> EGLEQLEAQTNFTKRELQVLYRGFKNECPSGVVNEDTFKQIYAQFFPHGDASTYAHYLFNAFDTTQTGSVKFEDFVTALSILLRGTVHEKLRWTFNLYDINKDGYINKEEMMDIVKAIYDMMGAYTYPVLAEDTPRQHVDVFFQKMDKNKDGIVTLDE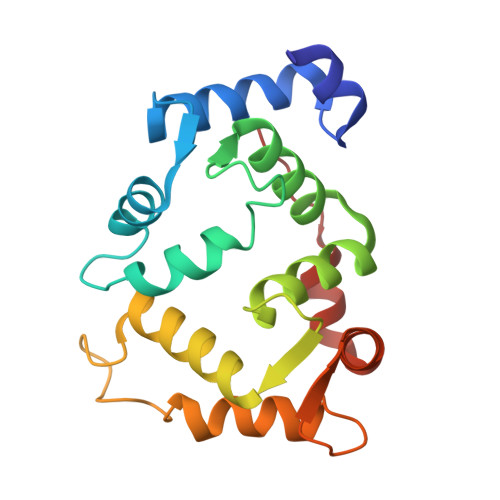FLESCQEDDNIMRSLQLFQNVM pmcRecently, Griffith-Jones and colleagues investigated the structural basis of RAD18 regulation by MAGEA4 through NMR titration and AlphaFold2 modeling to elucidate the interaction between the RAD6-binding domain (R6BD) of RAD18 and the MAGE homology domain (MHD) of MAGEA4. In our effort to develop peptide inhibitors targeting the RAD18-binding interface of the MHD of MAGEA4 (Fleming et al, 2023, Fleming et al, 2022), we determined the crystal structure of the MAGEA4 MHD/RAD18 R6BD complex at 2.58 Å resolution (statistics shown in Table EV1).

Each unit cell contains two protomers of the MAGEA4 MHD-RAD18 R6BD complex, with similar conformations. Protomer 1 (with the MAGEA4 MHD in chain A and the RAD18 R6BD in chain B) has slightly better quality and is used for analysis here. The electron density of the RAD18 R6BD (chain B) is very well defined in the map except for the sidechains of K347 and E349 located at N-terminal end of the R6BD helix (omit map shown in Fig. EV1). We found that the RAD18 R6BD forms a single α-helix and binds to a surface valley of the MAGEA4 MHD formed by helices α1, α3, α4, α5, and α8. Numerous interactions between the hydrophobic residues of the MAGEA4 MHD (M161, I162, F163, I205, M212, V239, V291, and V294) and RAD18 R6BD (A365, I364, Y361, A357, L353, and V354) are observed. Surprisingly, we found that the RAD18 R6BD peptide binds in the opposite orientation to the AlphaFold2 model presented by Griffith-Jones and colleagues (compare Fig. 1A with Griffith-Jones et al). Therefore, although the reported NMR perturbation and mutagenesis data appeared to be supporting the AlphaFold model, the interacting pairs of MAGEA4 and RAD18 residues are completely scrambled in the AlphaFold2 model in comparison with the experimental structure due to the flipped helix orientation of the RAD18 R6BD. The binding mode of a small peptide might be affected by crystal packing, and the MAGEA4-RAD18 R6BD complex might exist in solution with an alternative conformation or with multiple conformations. Our structural elucidation of the MAGEA4 MHD-RAD18 R6BD complex has provided molecular evidence to clarify confusions caused by the AlphaFold2 modeling and accelerate the development of MAGEA4-RAD18 antagonists to dismantle a key enabling feature of cancer cells.

>[2x]SNADAESLFREALSNKVDELAHFLLRKYRAKELVTKAEMLERVIKNYKRCFPVIFGKASESLKMIFGIDVKEVDPTSNTYTLVTCLGLSYDGLLGNNQIFPKTGLLIIVLGTIAMEGDSASEEEIWEELGVMGVYDGREHTVYGEPRKLLTQDWVQENYLEYRQVPGSNPARYEFLWGPRALAETSYVKVLEHVVRVNARVRIAYPSLREAALLEEEEGV;>[2x]HSKYRKKHKSEFQLLVDQARKGYKKIAG>[2x]SNAGNLSFLATSDGASLAYRLDGAAEKPLLALSNSIGTTLHMWDAQLPALTRHFRVLRYDARGHGASSVPPGPYTLARLGEDVLELLDALEVRRAHFLGLSLGGIVGQWLALHAPQRIERLVLANTSAWLGPAAQWDERIAAVLQAEDMSE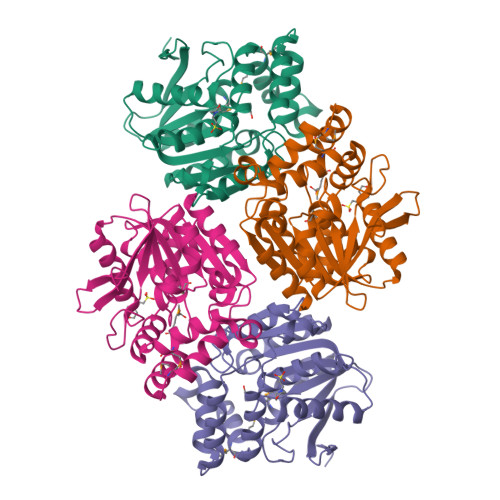TAAGFLGNWFPPALLERAEPVVERFRAMLMATNRHGLAGSFAAVRDTDLRAQLARIERPTLVIAGAYDTVTAASHGELIAASIAGARLVTLPAVHLSNVEFPQAFEGAVLSFLGA> GPAGRSIYNSFYVYCKGPCQRVQPGKLRVQCSTCRQATLTLTQGPSCWDDVLIPNRMSGECQSPHCPGTSAEFFFKCGAHPTSDKETSVALHLIATNSRNITCITCTDVRSPVLVFQCNSRHVICLDCFHLYCVTRLNDRQFVHDPQLGYSLPCVAGCPNSLIKELHHFRILGEEQYNRYQQYAAEECVLQMGGVLCPRPGCGAGLLPEPDQRKVTCEGGNGLGCGFAFCRECKEAYHEGECSAVFEASGTTTQAYRVDERAAEQARWEAASKETIKKTTKPCPRCHVPVEKNGGCMHMKCPQPQCRLEWCWNC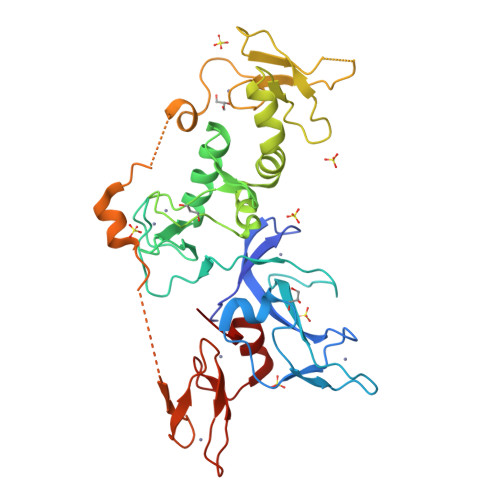GCEWNRVCMGDHWFDV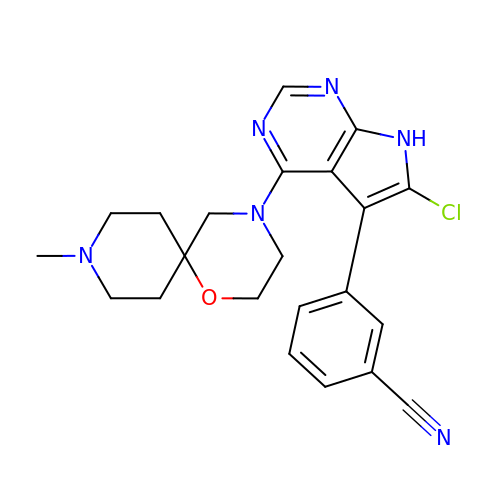(3P)-3-[6-chloro-4-(9-methyl-1-oxa-4,9-diazaspiro[5.5]undecan-4-yl)-7H-pyrrolo[2,3-d]pyrimidin-5-yl]benzonitrile | C22 H23 Cl N6 O | ZNRKSAWCBMXCBN-UHFFFAOYSA-N>MSHNIIEKKYRSNINDKIEQLRRTVPTLRVAYKKCNDLPITSRDLADLDGLEPATKLNKASILTKSIEYICHLERKCLQLSLANQHLSN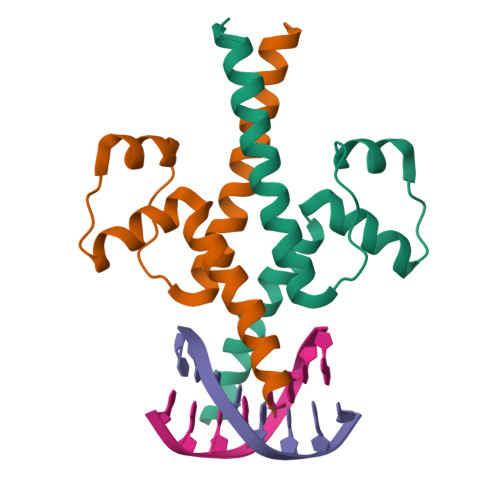DTRDSFVHLTEPSHHHHHH[6x]>[2x]MRGSHHHHHHENLYFQGSMLIDLITSYRKTAAIYTFVDAGLSIHFKNG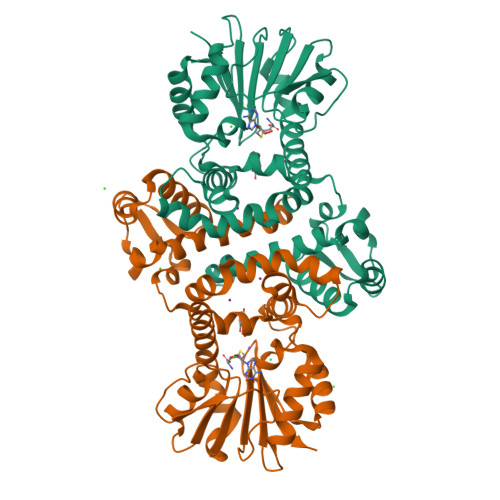DYVDINKLASQYGIDYSRLNRLCDFLIEIGVLVSSDHGVALSEECSALADPNSVEFLTVKYEINSEHWDSWLMYPKSLLENNGKSAFEMVHGKSFFEHLDSNKGLKSDFDALMSKYTNKIIKELLVIYDFDKHNRILDLGGGDGELLIRISEQVKGKDYTVLDRYNEVPISEGINFIKGDFFKPIPTGYDLYILKNVLHNWPDNDAISILKNCREAMDNNATLLIITLMKKPQSLVVKSVDILMDMLFSAKQRYLSEFEDIANQAGLVIRHYKDLDEIFSLIELKVK L-TYROSINAMIDE | C9 H12 N2 O2 | 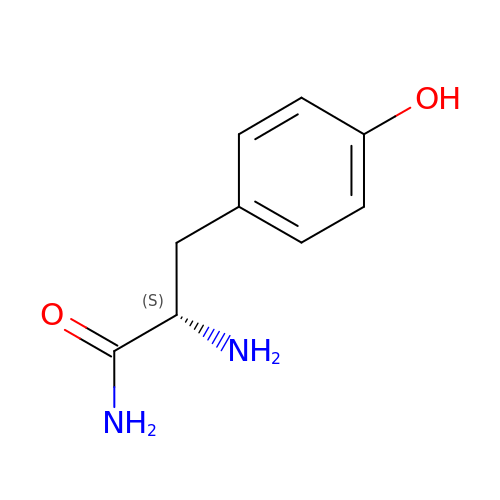PQFMNVGMJJMLAE-QMMMGPOBSA-N2-[(2-carboxyphenyl)amino]-5-[(5-phosphonopentyl)oxy]benzoic 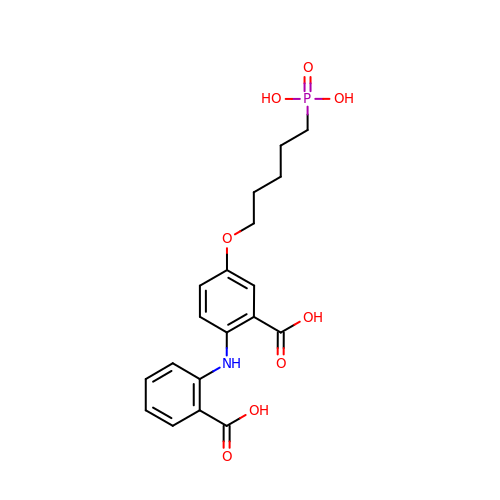acid | C19 H22 N O8 P | HYMLLKWKTLKWNS-UHFFFAOYSA-N Myosin VI is the only currently known unconventional myosin motor that transports cargoes along the actin filaments from the plus end to the minus end. As a unique myosin motor, Myosin VI can not only serve as a processive dimer or oligomer for vesicular transport and cargo sorting, but also function as a nonprocessive monomeric anchor or tether to link its binding cargoes with cytoskeletons for the establishment and maintenance of highly specialized cellular structures. A previous study revealed that Tom1 can directly interact with Myosin VI through its uncharacterized C-terminal region, and was proved to be a crucial adaptor to mediate endosomal localization of Myosin VI12. In this study, we systematically characterize the interactions of Myosin VI with Tom1 and three autophagy receptors, NDP52, TAX1BP1, and Optineurin, and discover that the C-terminal region of Tom1 contains a conserved Myosin VI-binding motif shared by all Tom1 family members, which can specifically interact with the C-terminal CBD of Myosin VI to form a stable heterodimeric complex.

We purified the C-terminal CBD of Myosin VI and Tom1 MBM complex, and successfully obtained good crystals that diffracted to 1.80 Å resolution. The overall structures of two complex molecules in the asymmetric unit are essentially the same, except that the flexible extreme N-terminal α-helix of Myosin VI in one complex molecule is unsolved due to the lack of electron density. In the complex structure, the C-terminal CBD of Myosin VI features an architecture assembled by a 4-stranded antiparallel β-sheet packing with five α-helices, and particularly, one surface of the 4-stranded β-sheet is covered by three helices (α3–α5), while the other side is capped by the short α2 helix. Intriguingly, Tom1 MBM in the complex structure mainly forms a continuous α-helix, and packs extensively with the solvent-exposed side of the 4-stranded β-sheet of Myosin VI containing the α2 helix (hereafter referred to as site I), burying a total of ~827 Å2 surface area. Further detailed structure analyses of the binding interface of Myosin VI/Tom1 complex revealed that the specific interaction between the C-terminal CBD of Myosin VI and Tom1 MBM is mainly mediated by extensive hydrophobic and polar interactions. In particular, the hydrophobic side chains of F444, F447, L448, and A452 of Tom1 occupy a hydrophobic groove formed by the side chains of I1173, F1175, W1193, C1227, L1229, T1234, and L1236 from Myosin VI, and concurrently, the hydrophobic side chains of Tom1 A454, A455, L458, P459, and L461 residues pack against a hydrophobic patch formed by the side chains of P1213 and I1215 together with the aliphatic side chain of K1212 from Myosin VI.

>[2x]ARQREIEMNRQQRFFRIPFIRPADQYKDPQSKKKGWWYAHFDGPWIARQMELHPDKPPILLVAGKDDMEMCELNLEETGLTRKRGAEILPRQFEEIWERCGGIQYLQNAIESRQARPTYATAMLQSLLK;>GVTSEGKFDKFLEERAKAADRLPNLSS[2x]>EQTAAPAKPVTVEAKNETFAPQHPDQYLSWKATSEQSERVDALAEDPRLVILWAGYPFSRDYNKPRGHAFAVTDVRETLRTGAPKNAEDGPLPMACWSCKSPDVARLIQKDGEDGYFHGKWARGGPEIVNNLGCADCHNTASPEFAKGKPELTLSRPYAARAMEAIGKPFEKAGRFDQQSMVCGQCHVEYYFDGKNKAVKFPWDDGMKVENMEQYYDKIAFSDWTNSLSKTPMLKAQHPEYETWTAGIHGKNNVTCIDCHMPKVQNAEGKLYTDHKIGNPFDNFAQTCANCHTQDKAALQKVVAERKQSINDLKIKVEDQLVHAHFEAKAALDAGATEAEMKPIQDDIRHAQWRWDLAIASHGIHMHAPEEGLRMLGTAMDK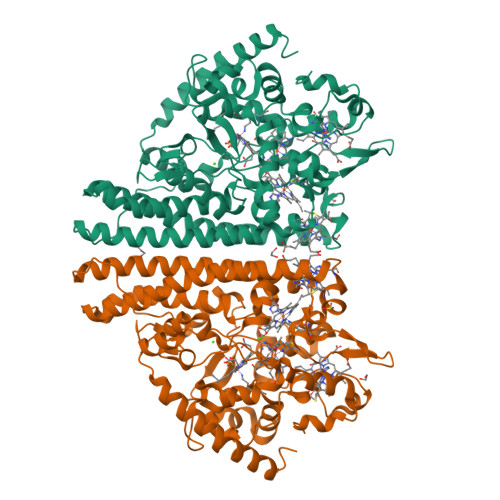AADARTKLARLLATKGITHEIQIPDISTKEKAQQAIGLNMEQIKAEKQDFIKTVIPQWEEQARKNGLLSQ[4x]2-amino-8-[2-oxo-2-(4-phenylphenyl)ethyl]sulfanyl-1,9-dihydropurin-6-one 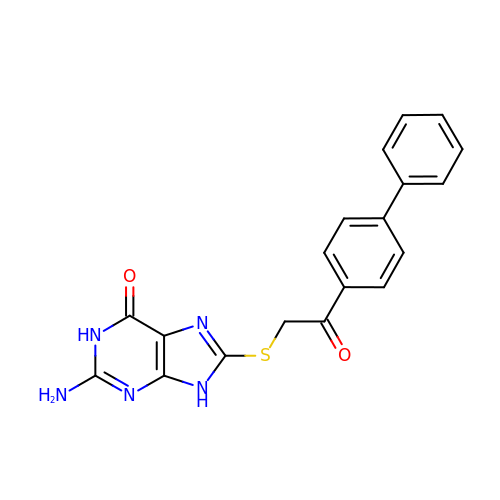| C19 H15 N5 O2 S | JPQMPGXXKRYOGX-UHFFFAOYSA-N>GMDKSAKAPAITIFDHRGCSRAPKESSAKSGSQDDEMLVKVASTKVTVSEDVAAKKLQEFIGFKEKGLDGSVIRKK[4x];>[8x]MLDAFSRVVTNADSKAAYVGGADLQALKKFISEGNKRLDAVNSIVSNASCIVSDAVSGMICENPSLISPSGNCYTNRRMAACLRDAEIILRYVSYALLSGDSSVLEDRCLNGLKETYSSLGVPANGNARAVSIMKACSVAFVNNTASQKKLSTPQGDCSGLASEVAGYFDKVTSAIS;>[4x]AMDKSAKAPVITIFDHRGCSRAPKEYTGSKASGQDDEMMVKAQSVKIAVSDGVAESVLKDSL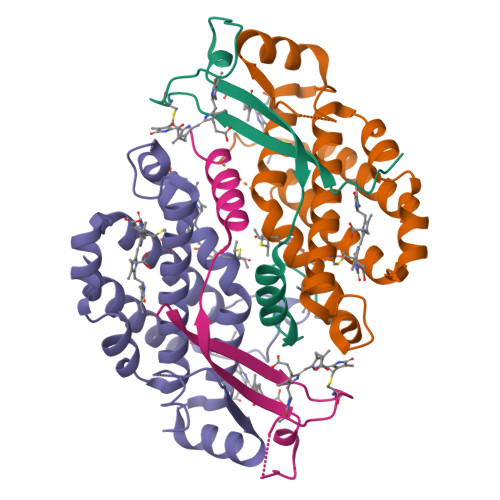SVMHK>GAMSQPPKWTTSNGAPVSDVFATERATFDNANHANNAPKVGPLLLQDFQLIDSLAHFDRERIPERVVHAKGAGAFGEFEVTDDISDVCAAKFLDTIGKKTRIFTRFSTVGGEKGSADSARDPRGFSTKFYTEEGNLDLVYNNTPIFFIRDPSKFPHFIHTQKRNPATNLKDANMFWDYLVNNQESIHQVMYLFSDRGTPASLRKMNGYSGHTYKWYNKKGEWVYVQVHFKSDLGVVNFNNEEAGKLAGEDPDYHTGDLFNAIERGEYPSWTCYIQTMTQEQAAKQPFSVFDLTKVWPHKDFPLRRFGKFTLNENPKNYFAEVEQAAFSPSHTIPSMQPS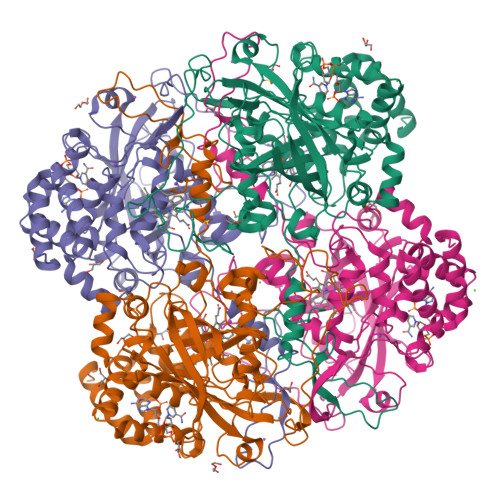ADPVLQSRLFSYPDTHRHRLGVNYQQIPVNCPVAPVFTPQMRDGSMTVNGNLGSTPNYKSSFCPFSTEAQIQTNSHTPEEVLAAHTEKFHWGGILDSKSYDFEQPRALWKVFGKTPGQQRNFCHNVAVHVAAANHEIQDRVFEYFSKVYPEIGDQIRKEVLQLSPRGDSAARL[4x]>[2x]KSASLPPVNTDIHDWVKTKGAWDKGYKGQGKVVAVIDTGIDPAHQSMRISDVSTAKVKSKEDMLARQKAAGINYGSWINDKVVFAHNYVENSDNIKENQFEDFDEDWENFEFDAEAEPKAIKKHKIYRPQSTQAPKETVIKTEETDGSHDIDWTQTDDDTKYESAGMHVTGIVAGNSKEAAATGERFLGIAPEAQVMFMRVFANDVMGSAESLFIKAIEDAVALGADVINLSLGTANGAQLSGSKPLMEAIEKAKKAGVSVVVAAGNERVYGSDHDDPLATNPDYGLVGSPSTGRTPTSVAAINSKWVIQRLMTVEELEKRADLNHGKAIYSESVDFKNIKDSLGYDKSHQFAYVKESTDAGYNAQDVKGKIALIERDPNKTYDEMIALAKKHGALGVLIFNNKPGQSNRSMRLTANGMGIPSAFISHEFGKAMSQLNGNGTGSLEFDSVVSKAPSQKGNEMNHFSNWGLTSDGYLKPDITAPGGDIYSTYNDNHYGSQTGTAMASPQIAGASLLVKQYLEKTQPNLPKEKIADIVKNLLMSNAQIHVNPETKTTTSPRQQGAGLLNIDGAVTSGLYVTGKDNYGSISLGNITDTMTFDVTVHNLSNKDKTLRYDTELLTDHVDPQKGRFTLTSRSLKTYQGGEVTVPANGKVTVRVTMDVSQFTKELTKQMPNGYYLEGFVRFRDSQDDQLNRVNIPFVGFKGQFENLAVAEESIYRLKSQGKTGFYFDESGPKDDIYVGKHFTGLVTLGSETNVSTKTISDNGLHTLGTFKNADGKFILEKNAQGNPVLAISPNGDNNQDFAAFKGVFLRKYQGLKASV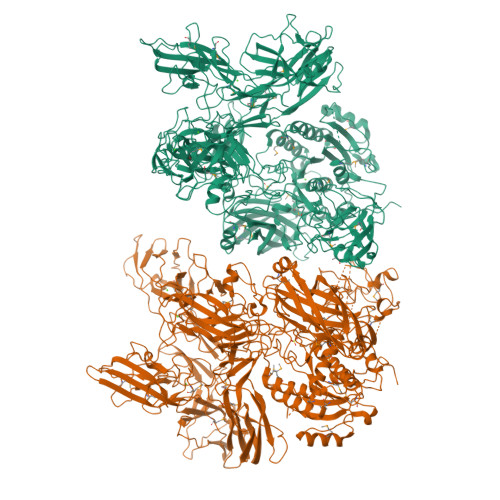YHASDKEHKNPLWVSPESFKGDKNFNSDIRFAKSTTLLGTAFSGKSLTGAELPDGYYHYVVSYYPDVVGAKRQEMTFDMILDRQKPVLSQATFDPETNRFKPEPLKDRGLAGVRKDSVFYLERKDNKPYTVTINDSYKYVSVEDNKTFVERQADGSFILPLDKAKLGDFYYMVEDFAGNVAIAKLGDHLPQTLGKTPIKLKLTDGNYQTKETLKDNLEMTQSDTGLVTNQAQLAVVHRNQPQSQLTKMNQDFFISPNEDGNKDFVAFKGLENNVYNDLTVNVYAKDDHQKQTPIWSSQAGAGASAIESTAWYGITARGSKVMPGDYQYVVTYRDEHGKEHQKQYTISVNDKKPMITQGRFDTINGVDHFTPDKTKALGSSGIVREEVFYLAKKNGRKFDVTEGKDGITVSDNKVYIPKNPDGSYTISKRDGVTLSDYYYLVEDRAGNVSFATLRDLKAVGKDKAVVNFGLDLPVPEDKQIVNFTYLVRDADGKPIENLEYYNNSGNSLILPYGKYTVELLTYDTNAAKLESDKIVSFTLSADNNFQQVTFKMTMLATSQITAHFDHLLPEGSRVSLKTAQGQLIPLEQSLYVPKAYGKTVQEGTYEVVVSLPKGYRIEGNTKVNTLPNEVHELSLRLVKVGDASDSTGDHKVMSKNNSQALTASATPTKTTTPATAKALPSTGEKMGLKLRIVGLVLLGLTCVFSRKKSTKD(2~{S})-1-[2,4-bis(chloranyl)-3-[[2-methyl-4-(trifluoromethyl)quinolin-8-yl]oxymethyl]phenyl]carbonyl-~{N}-methyl-pyrrolidine-2-carboxamide | C25 H22 Cl2 F3 N3 O3 | 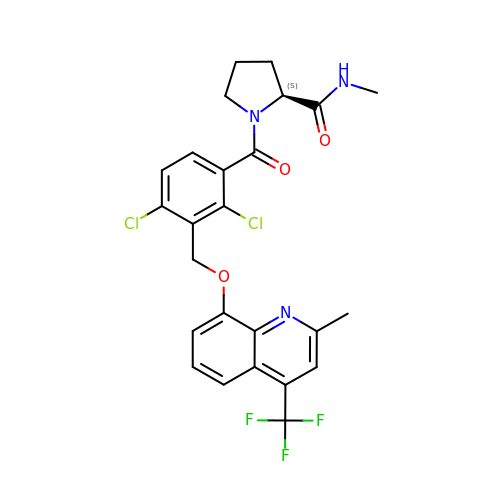SGDYSAAUPQPUSM-IBGZPJMESA-N>GIDPFTESVLQSQATELLQKKAQLVSFKIQGIMKRIFMGANTLEKFLSDENSAINDTLKRRMLSEFLLANPHVLLVSAIYTNNNERVITAMSMDSKIAYPNTTLNENMTNQIRSLKSITHSDPYYKEVNGDKIYGMDITLPLMGKNQNAIGALNFFLNIDAFYTDVVGKKKSNTFLMGKDGRLLINPNREIQDKILSAINPDRRVAKAVEYYNQNEAGTLSYHSLSGNTETFLAIQPFDFFEEKGNNGNHWRWAIGKYVNKSLVFKEATN[3x]

Extracellular chemicals are sensed by chemoreceptors, also termed transducer-like proteins (Tlps). Most of the characterised Tlps are dimeric membrane proteins that comprise an extracytoplasmic ligand-binding domain (LBD), the transmembrane region, the HAMP (histidine kinases, adenylyl cyclases, methyl-accepting protein, and phosphatases) domain and the methyl-accepting (MA) domain, the latter transmitting information to a signalling cascade. H. pylori tlpC mutants are outcompeted by wild type during stomach colonisation, and TlpC modulates the chemotactic response to acid. In common with family 1 histidine kinases, the TlpC LBD has a dCACHE fold, and is composed of a membrane-proximal and membrane-distal PAS-like modules folding against the N-terminal and C-terminal halves of a long stalk helix, respectively.

In this paper, we report the crystal structure of LBD of H. pylori TlpC in complex with a small-molecule ligand that co-purified with the protein. The three-dimensional structure of recombinant H. pylori TlpC LBD (residues 34–297 plus six additional residues (GIDPFT) at the N-terminus, introduced as an artifact of the cloning procedure), was determined by X-ray crystallography using a single-wavelength anomalous dispersion (SAD) technique to a resolution of 2.2 Å. The TlpC LBD crystals (hereafter referred to as form A) belonged to the space group C2, with three molecules in the asymmetric unit related to each other by a three-fold pseudo-symmetry. The ligand was bound to the membrane-proximal subdomain. Based on the analysis of the electron density maps and the chemical nature of the ligand-binding pocket, we hypothesised and confirmed the ligand to be lactate. The lactate binding site is located in a pocket formed by residues F202, L210, N213, I218, L223, Y249, L252, S253, and Y285. The carboxyl and hydroxyl groups of lactate form hydrogen bonds with the side chains of N213, Y249 and Y285, and with the main-chain amides of L252 and S253. The TlpC LBD/lactate complex is further stabilised by hydrophobic interactions between the methyl group of lactate and the side chains of F202, L210, I218 and L223. ITC measurements demonstrated that each of the N213A, I218A, Y285A and Y249F substitutions abolished the binding of lactate to TlpC LBD. Our analysis of the structural basis of lactate recognition by H. pylori chemoreceptor TlpC changes this paradigm regarding the mechanism of sensing by dCACHE domain by providing the first example where direct sensing of the signal molecule is mediated by the ligand binding to the membrane-proximal, rather than membrane-distal, subdomain.> GPLPNKLWCICRQPHNNRFMICCDLCEDWFHGTCVGVTKAMGTDMENKGIDWKCPKC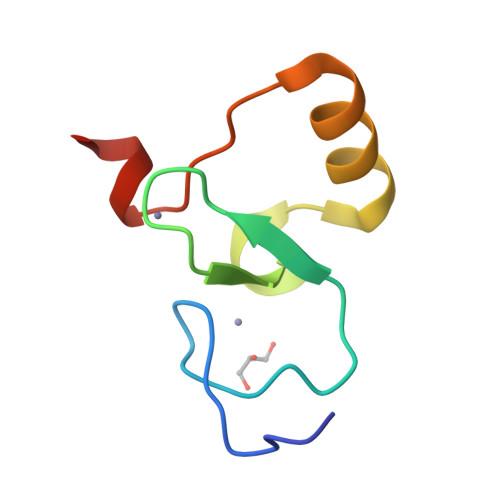VKRQE>[4x]DQNFARNEKEAKDSAITFIQKSAAIKAGARSAEDIKLDKVNLGGELSGSNMYVYNIST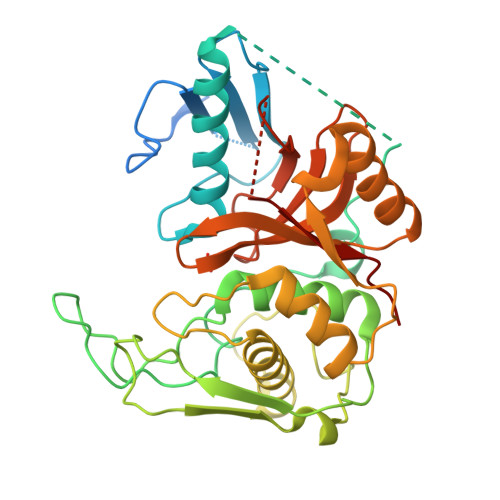GGFVIVSGDKRSPEILGYSTSGSFDVNGKENIASFMESYVEQIKENKKLDSTYAGTAEIKQPVVKSLLDSKGIHYNQGNPYNLLTPVIEKVKPGEQSFVGQHAATGSVATATAQIMKYHNYPNKGLKDYTYTLSSNNPYFNHPKNLFAAISTRQYNWNNILPTYSGRESNVQKMAISELMADVGISVDMDYGPSSGSAGSSRVQRALKENFGYNQSVHQINRGDFSKQDWEAQIDKELSQNQPVYYQGVGKVGGHAFVIDGADGRNFYHVNWGWGGVSDGFFRLDALNPSALGTGGGAGGFNGYQSAVVGIKP>GSHMDASVMSTTYALSAAQTEIWLAQQLYPDSPVYNIAQYTVIEGVIEPAVFEAALRQVIDEADTLRLQFIDSDDGLRQRIGTPAWSMPVLDLTAQADPQAAAQAWMRADYQQPVNLTQGPLFCYALLKVAPAQWMWYQRYHVIMMDGYGAYLIAQRVAYVYSALCEGTTPAECDFGSILQLLESDAQYQISAQRAQDEAYWLKHCANWSEPATLASRSAPVLQQRLRQTTYLAIQALGDTAPDARRLAQFMTAAMAAYLYRFTGEQDVVLGLPVKVRFGADRHIPGMKSNTLPLRLTMRPGMNLSSLMQQAAQEMQSGLRHQRYPSEALRRQLGMPSGQRLFGTTVNVMPFDLDLSFGGYSATNHNLLNGPAEDLMLGVYWTPGSHQLRIDFDANPACYTPEGLGAHQRRFIRFMQVLAADATQPIDSIDLLD[4x]

Nonribosomal peptide synthetases (NRPSs) are multimodular enzymes that catalyze the biosynthesis of diverse peptides with a wide variety of activities. The incorporation of an acyl into peptidyl backbone is usually implemented by a starter condensation (Cs) domain, normally located at the beginning of the initial NRPS module, via the formation of an amide bond to the α-amino group of the first amino acid residue, a process also known as lipoinitiation. Genome mining of two Cs domain-embedded cryptic NRPS biosynthetic gene clusters, rzmA and holA, in the bacterium P. rhizoxinica HKI 454 resulted in the discovery of two distinct types of lipopeptides, cyclic rhizomide A (1) containing an uncommon acetyl chain (C2) and linear holrhizin A (2) harboring a medium octanoyl (C8) chain. Similar to other C domain structures reported previously, RzmA-Cs adopts a “V-shaped” configuration and consists of two subdomains (N- and C-lobes) each representing the chloramphenicol acetyltransferase (CAT) fold.

To diminish the reaction rate, we made an additional mutation on the second histidine of the “HHxxxDG” motif37 of RzmA-Cs R148A to create the double mutant H140V/R148A, which finally enabled us to obtain several crystals in the absence or presence of substrates. We then solved and analyzed these H140V/R148A structures. The overall structure of unbound H140V/R148A is almost identical to the structures of WT and R148A in both conformations. Thus, the H140V mutation did not completely abolish the condensation activity, correlating well with its role in substrate positioning. Based on these H140V/R148A structures and related functional assays, we propose three potential conformational states (i.e., “unbound-bound-released”) within the lipoinitiation reaction cycle catalyzed by Cs domains. The major conformational changes during this cycle reflect the relative positions of two lobes, in concert with the binding of substrates and release of products.> M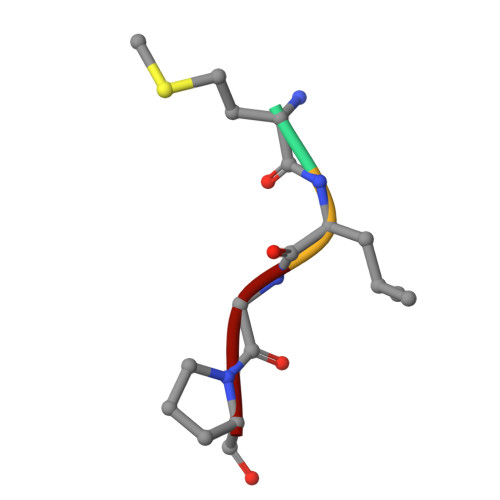LGP>[2x]MGSSHHHHHHSSGLVPRGSHSDEVDAHMSVASAVEVGVGEDEEEGVEEEEEEVEAVVMPERYALGGACRVLAGMPAPLGATALDGGVNFAVYSAGASAASLCLFTPDDLEADEVTEEVPLDPLFNRTGNVWHVFIEGELHNMLYGYRFDGMFAPHCGQYFDVSNVVVDPYAKAVISRGEYGVPGPGGDCWPQMAGMIPLPYSTFDWQGDLPLRYPQKDLVIYEMHLRGFTKH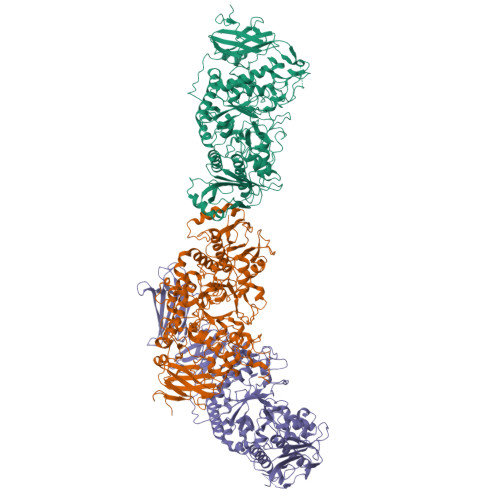SSSNVEHPGTYIGAISKLDYLKELGVNCVELMPCHEFNELEYFSCSSKMNFWGYSTINFFSPMIRYSSGGIRNCGRDAINEFKTFVREAHKRGIEVIMDVVFNHTAEGNEKGPILSFRGIDNSTYYMLAPKGEFYNYSGCGNTFNCNHPVVREFIVDCLRYWVTEMHVDGFRFDLASIMTRGCSLWDPVNVYGSPVEGDMTTTGTPLATPPLIDMISNDPILGDVKLIAEAWDAGGLYQVGQFPHWKIWSEWNGKYRDIVRQFIKGTDGFAGGFAECLCGSPHLYQAGGRKPWHSINFVCAHDGFTLADLVTYNKKYNSSNGEDNRDGENHNLSWNCGEEGEFAGLSVKRLRKRQMRNFFVSLMVSQGVPMFYMGDEYGHTKGGNNNTYCHDHYVNYFRWDKKEESSDLQRFCSLMTKFRKQCESLGLADFPTAQRLHWHGHQPGKPDWSETSRFVAFSTKDETKGEIYVAFNASHLPAVVGLPERPGYRWEPLVDTGKPAPYDFLTDDLPDRAHAVHLFSHFLNSNLYPMLSYSSIILELQPDD;> MASLPAPPTPLGSCPRGRGGGRVVARPRRAGLACAARSCYRFRTDDDGVVDVAVSGEDGDGGGGGYAVSVEVPGTRGREGGLVLRASGSGEGVPLAPAAGGASLAAELSFDPTRAPFYLSFLLTDASGAEIRTHRKTSFRVPVGVGPGSPAPLGMSISGDGAVNFAVYSKNANAVSLYLYAAAVGGGGGDEPALEIDLDPYIHRTGNVWHVSLASVDGYVSYAFCCGGIRRPLLDPYAKVIGDFVSSNSVYDEGVTAPSMRCFASLAIAPSYNWGRDRHPRLPLEKLVVYRANVALFTKDRSSGLPDDAAGTFTGLSAKVEHFRSLGVNAILLEPVFPFHQVKGPYFPYHFFSPMNLYSSKGLSVSAIKSMKDMVRVMHRNGIEVLLEVVFTHTAEGESECQTISMRGIDNSSYYIANGIAGCKASILNCNHPVTQKLILDSLRHWVLDFHVDGFCFINAPFLVRGPGGEYLSRPPLLEAITFDPVLSMTKIIADPWSPLDISNVQFPFPHWKRWAEVNTRFSIDVRKFLKREALISDLATRLCGSGDLFSTRGPAFSFNHVSRNSGLSLVDLVSFSNDDLLSESSWNCGEEGPSENSAVLQTRLRQIRNFLFILFVSLGVPVLNMGDECGHSAAGSVSYKDRGPLNWRGMKTTFVKEVTGFISFLTALRSRRGDIFQRREFLKLENIHWYGSDLCEPGWDDPTSNFLCMHINAEVDEMAADSVRGDLYICFNANEESVSAALPALAEGSVWLRLVDTSLAFPGFFATESNPKVQQVPGLSSYHVEAHTCVLFESKSALA>[4x]SSVPTVKLFIGGKFVESKSDKWIDIHNPATNEVIGRVPQATKAEMDAAIASCKRAFPAWADTSVLSRQQVLLRYQQLIKENLKEIAKLITLEQGKTLADAEGDVFRGLQVVEHACSVTSLMMGETMPSITKDMDLYSYRLPLG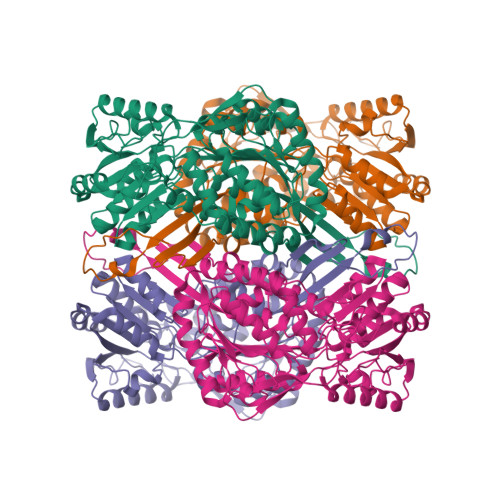VCAGIAPFNFPAMIPLWMFPMAMVCGNTFLMKPSERVPGATMLLAKLLQDSGAPDGTLNIIHGQHEAVNFICDHPDIKAISFVGSNKAGEYIFERGSRHGKRVQANMGAKNHGVVMPDANKENTLNQLVGAAFGAAGQRCMALSTAVLVGEAKKWLPELVEHAKNLRVNAGDQPGADLGPLITPQAKERVCNLIDSGTKEGASILLDGRKIKVKGYENGNFVGPTIISNVKPNMTCYKEEIFGPVLVVLETETLDEAIQIVNNNPYGNGTAIFTTNGATARKYAHLVDVGQVGVNVPIPVPLPMFSFTGSRSSFRGDTNFYGKQGIQFYTQLKTITSQWKEEDATLSSPAVVMPTM>MGNVIDLGEYGARFTEDPYPVYAELRERGPVHWVRTPPPEAFEGWLVVGHEEARAALADPRLSKDGTKKGLTSLDVELMGPYLLVVDPPEHTRLRSLVARAFTMRRVEALRPRIQEITDGLLDEMLPRGRADLVDSFAYPLPITVICELLGVPDIDRVTFRALSNEIVAPTGGDAELAAYERLAAYLDELIDDKRSTAPADDLLGDLIRTRAEDDDRLSGEELRAMAFILLVAGHETTVNLIT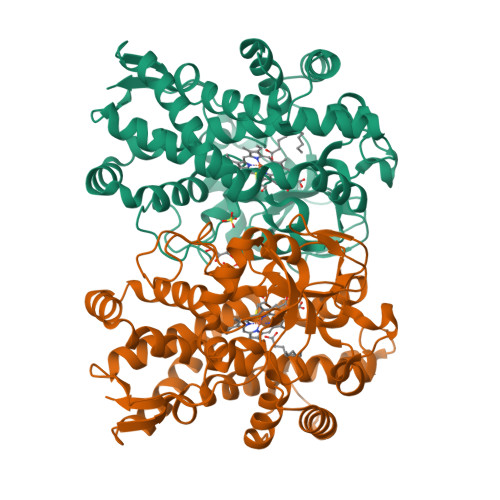NGVHTLLTHPDQLAALRADMTLLDGAVEEVLRFEGPVETATYRYAAESMEIGGTAIAEGDPVMIGLDAAGRDPARHPDPHVFDIHRAPQGHLAFGHGIHYCLGAPLARLEARVALRSLLERCPDLALDGPPGARPPGMLIRGVRRLPVRW[2x]>KAPPLVNLAEEKDVKVTVGENMDLKNADLLTDGDKYYLQHDATGNKEGNNWENYQEQGTEVTSTAEGKNGVWVQVDLGASYPLEVINLKRQVYDGQATIGNGNPSGQGKRLKGTKISYKNTAIVIGNEEDLSDGQIVYYEGNPTLPDGVKQPENVSKPYEEAMGGQWFYMDYANKNGLGATELGTTKEARYIRVYTENPKGAAVKFMELGIYGYENEQDVQSQDGPRRVIDNEHPMMIATAYSNDVYEIGQEEGPELQGSNTVDGRWNAIPDDLKENNVLLLHTNNLRQFAPDHIGQAYLQAFHEHGLQIAYEQGAPIMLLGLTAAATPENGGTQYNITADMDYGWLDLMYRMYPNMQGVFNTENFWAGIHPPCEGSAKMLEIADRFGGFFVWSDQDHGSTVTNIVSNANMKKALEKHGDAFYLIYKNTSSNQPDDLKTSSFFQGSWLAGYTGGWGMLSDTWAWDKQFSKLWQGAGSYNNWQRLCGEPEALLGMQMMSTYLGGGVIYTFEFPEIVYGTSNTNSPANTHVLTELFRYIVNHPAPSKKEIMEETKAVLYGNVSSDFYSGLSGKPTGFQIYETGRYGIIPVIPTWGTRAEVTKKLIQEADKLGVTPPNVLDVKDKNLSGQAKQKYFKDLYPIEYVGNAFADKWEGTWYLYNNKVNTNEKQHAILPLEGEEESARLKVEMEPHEFMIMNESGDGTAMDITLNNYRVNKDEIIFDNKFGLTWTGDFSPGQTTINGKLSVYKYMDEYNVVNAPEGKLSPEDNELRTTTFELTKLAK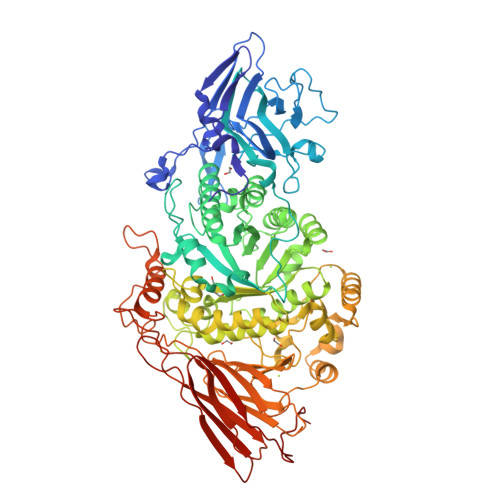EPKVQVVKGQQPDTDGQPQYTEPKVEFNEETGKAVITIQTNGWVDLSITGLEFVYDENAQKIEDEPIKS[2x]Recently our laboratory has introduced a powerful mode of photochemistry into proteins, namely triplet energy transfer (EnT) photocatalysis, by developing an enantioselective [2 + 2] cyclase that relies on a genetically programmed benzophenone as a triplet sensitizer. Compared with benzophenones, thioxanthones have strong absorbance features that extend into the visible spectrum and are less susceptible to off-pathway processes that compromise EnT efficiency. Here, we develop engineered translation components to embed thioxanthone triplet sensitizers into proteins. This system enables the development of highly efficient and oxygen-tolerant photoenzymes that are powered by visible light and can achieve selective conversions that are beyond the reach of existing photocatalysts.

To identify a suitable starting point for enzyme engineering, we elected to reposition the thioxanthone sensitizer to position 244 to create a larger active site pocket to accommodate the sterically demanding substrate 2. After screening ∼3,200 clones, an optimized SpEnT1.3 variant was identified containing six mutations clustered around the active site (P23C, Y37A, Y121G, G226L S271C, H287L) that achieves a sixfold improvement in reaction yield (78% with SpEnT1.3 versus 13% with SpEnT1.0). SpEnT1.3 also displays a high degree of stereocontrol, preferentially affording (S,S)-2a with 99% e.e. and 22:1 d.r. Notably, improvements in photoenzyme efficiency and stereocontrol across evolution also coincided with a substantial reduction in side-product formation, with only ∼5% of 3 and 4 formed with SpEnT1.3. Despite promoting more challenging chemistry, detailed characterization of SpEnT1.3 reveals that this photoenzyme exhibits impressive kinetic properties that are in line with the thioxanthone-containing [2 + 2] cyclase VEnT1.3, with a kcat of 8.7 ± 0.64 s−1 (at 100% light intensity), a Km of <15 µM and a total turnover number of >300 under aerobic conditions. A 1.8-Å resolution structure of SpEnT1.3 shows how the active site pocket has been extensively remodelled as a result of sensitizer repositioning and the mutations installed during evolution, leading to a substantial increase in active site volume. Molecular docking of (S,S)-2a reveals a productive binding pose with the ligand occupying a tight binding pocket lined by Cys23, Pro36, Ile72, Met90, Gln195, Leu226, Cys271 and Leu287. Similar to VEnT1.3, the quinolone ring of the ligand lies in close proximity to the mTX sensitizer with its carbonyl forming a hydrogen bond with the Gln195 side chain, consistent with a reaction mechanism involving energy transfer from the excited sensitizer to the substrate. Mutation of Gln195 to Ala leads to a fourfold decrease in activity, confirming its importance to SpEnT1.3 photocatalysis.

> MEIPVIEPLFTKVTEDIPGAAGCVFDKNGDFYIVAPAVEVNGKPAGEILRIDLKTGKKTVICKPEVNGYGGIPAGCQCDRDANQLFVADMRLGLLVVQTDGTFEEIAKKDSEGRRMQGCAGCAFDYEGNLWITAPAGEVAPADFTISLQEKFGSIYCFTTDGQMIQVDTAFQAPAGIAVRHMNDGRPYQLIVAEQPTKKLWSYDIKGPAKIENKKVWGHIPGTHKLGAAGMDFDEDNNLLVANXGSSHIEVFGPDGGQPKMRIRCPFEKPCALHFKPQTKTIFVTELENNAVWKFEWQRNGKKQYCETLKFGIFGSLEWSHPQFEK>[6x]GMYANKVKKIAAVHDLSGMGRVSLTVVIPILSSMGFQVCPLPTAVLSNHTQYPGFSFLDLTDEMPKIIAEWKKLEVQFDAIYTGYLGSPRQIQIVSDFIKDFRQPDSLIVADPVLGDNGRLYTNFDMEMVKEMRHLITKADVITPNLTELFYLLDEPYKADSTDEELKEYLRLLSDKGPQVVIITSVPVHDEPHKTSVYA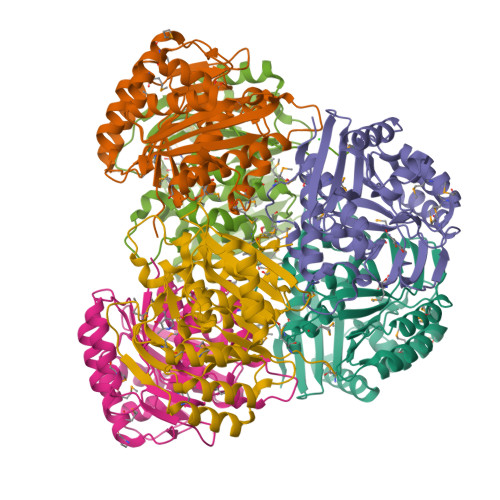YNRQGNRYWKVTCPYLPAHYPGTGDTFTSVITGSLMQGDSLPMALDRATQFILQGIRATFGYEYDNREGILLEKVLHNLDMPIQMASYELI> MLQPVFTLKLRHKISPRMVAVGRYDGTHPCLAAATQAGKVFIHNPHSRSQHLGAPRVLQSPLESDVSLLNINQTVSCLTAGVLNPELGYDALLVGTQTNLLAYDVYNNSDLFYREVADGASAIVLGTLGDITSPLAIIGGNCALQGFNHEGNDLFWTVTGDNVHSLALCDFDGDGKKELLVGSEDFDIRVFKEDEIVAEMSETEIITSLCPMYGSRFGYALSNGTVGVYDKTARYWRIKSKNQAMSIHAFDLNSDGVCELITGWSNGKVDARSDRTGEVIFKDNFSSA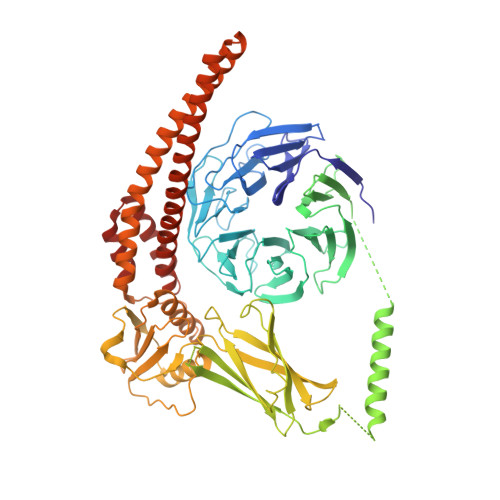IAGVVEGDYRMEGCQQLICCSVDGEIRGYLPGTAEMRGNLMDISVEQDLIRELSQKKQNLLLELRNYEENAKAELSSPLNEADGHRGVIPANTKHHTALSVSLGSEAQAAHAELCISTSNDTIIRAVLIFAEGVFAGESHVVHPSVHHLSSSVRIPITPPKDIPVDLHLKTFVGYRSSTQFHVFELTRQLPRFSMYALTSPDPASEPLSYVNFIIAERAQRVVMWLNQNFLLPEDTNIQNAPFQVCFTSLRNGGQLYIKIKLSGEITVNTDDIDLAGDIIQSMASFFAIEDLQVEADFPVYFEELRKVLVKVDEYHSVHQKLSADMADNSNLIRSLLVQAEDARLMRDMKTMKNRYKELYDLNKDLLNGYKIRCNNHTELLGSLKAVNQAIQRAGHLRVGKPKNQVITACRDAIRSNNINMLFRIMRVGTASS> SPSQSNGQDISLSCGASEPAVDQDKKKWEPDTKFLKTPNTVHAPATYQDPSLLSTVPYMTSRIFTAPATYEIPVKGDKRHMLRLHFYPSTYTGLNILDSYFSVAANDLTLLSNFSAAITCQALTQAYLVREYSLAPSEKDVLSIIFTPSDKHPKAFAFINGIEVIPMPELFDTASLVGFSDQTSDTKTANLQTM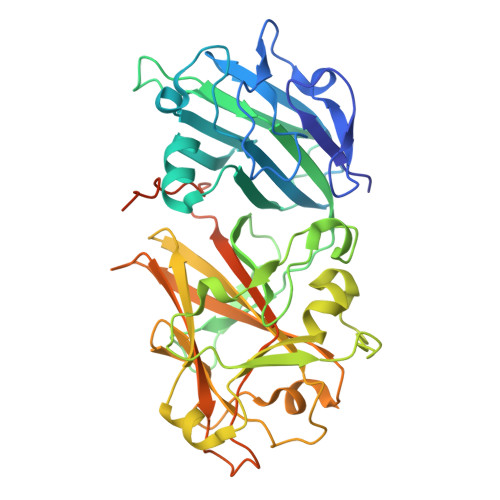FRLNVGGQDIPGSQDSGGLTRTWYNDAPYIFSAGLGVTLQASNNFRIDYQKMPVSTAPADVYKTARSQGPNGDINMKSNLTWMFQVDTNFTYIMRLHFCEFQLAKINQKVFNIFINNRTAQGDTNPADILGWTGGKGIPTYKDYAIYVDANTGGGGEEISLQMTPSTFGQPEYYDSQLNGLEIFKIDTMKNLAGPNPKPSPMQANEDVKKDFQGDKRITAFVIGSAGGVAAVLFCA(2~{R},3~{R},4~{R},5~{R})-3-acetamido-2-[(1~{R})-1,3-bis(oxidanyl)propyl]-5-fluoranyl-4-oxidanyl-2,3,4,5-tetrahydropyran-1-ium-6-carboxylic 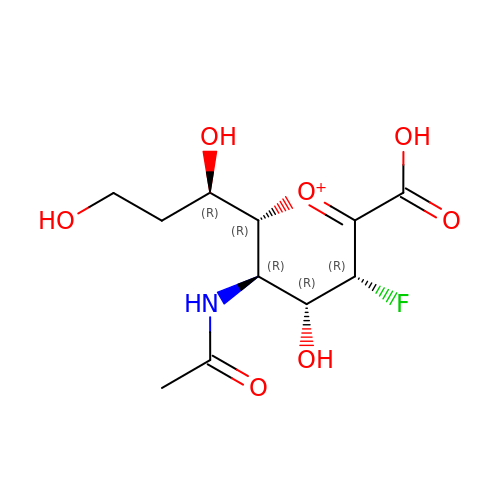acid | C11 H17 F N O7 | CHPKCUSAUNABPC-HXLXBVJFSA-O>[4x]MSLIRSATKEDGQAIARLVLVILKDMELPILEEVSEEQMIDLLAEATAYPTYRYGYQRILVYEHAGEVAGIAVGYPAEDEKIIDEPLREVFKKHGLAEDVRLFIEEETLPNEWYL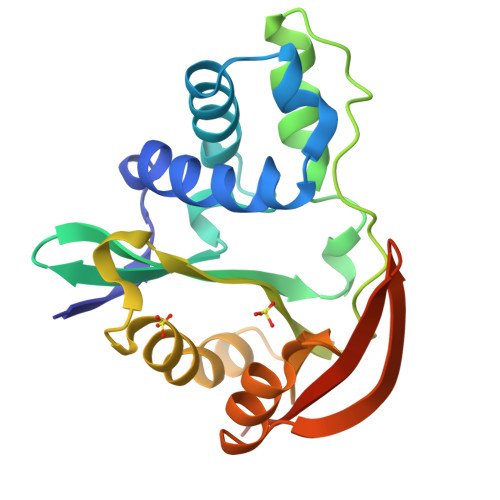DTISVDERFRGMGIGSKLLDALPEVAKASGKQALGLNVDFDNPGARKLYASKGFKDVTTMTISGHLYNHMQKEVEGGSHHHHHH4-{5-[(2E)-but-2-en-2-yl]thiophen-2-yl}-N,N-dimethylaniline 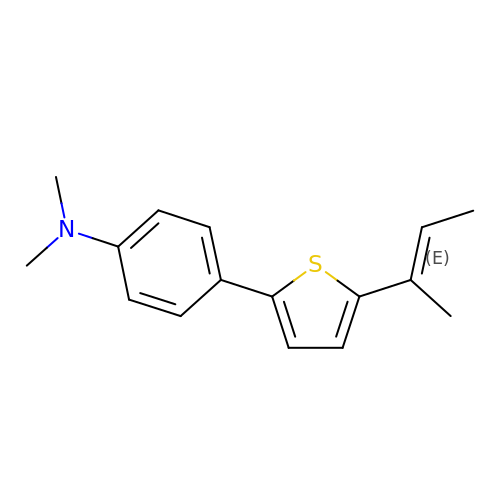| C16 H19 N S | AMMZMSCAYJQWSM-LFYBBSHMSA-N>[3x]GPLGSKPYECYICHARFTQSGTMKMHILQKHTENVAKFHCPHCDTVIARKSDL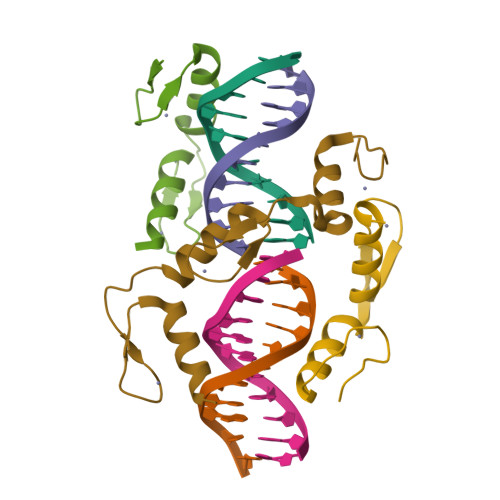GVHLRKQHSYIEQGKKCRYCDAVFHERYALIQHQKSHKNE> DKMPDWNIPSLYESYKNDFRIGVAIPAKCLSNDTDRRMVLKHFNSITAENEMKPESLLAGQTSTGLNYRFSTADTFVDFANTNNIGIRGHTLVWHSQTPDWFFKDSSGQRLTKDALLARLKQYIYDVVGRYKGKVY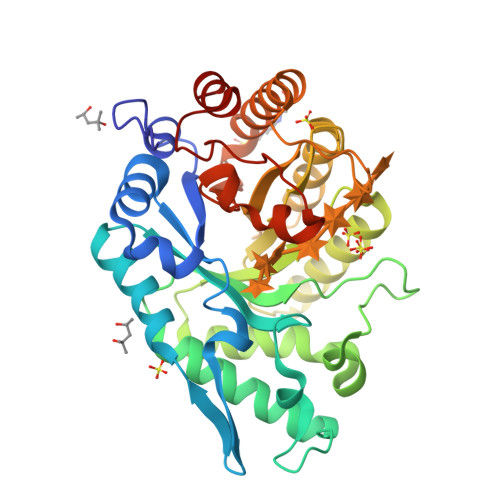AWDVVNQAIDENQSDGYRRSTWYEICGPEYIEKAFIWAHEADPNAKLFYNDYNTEISKKRDFIYNMVKNLKSKGIPIHGIGMQCHINVNWPSVSEIENSIKLFSSIPGIEIHITQLDMSLYNYGSSENYSTPPQDLLQKQAQKYKELFTMLKKYTNVVKCVTFWGLKDDYSWLRSFNGKNDWPLLLFEDYSAKPAYWAVIEAS> RERIPVEADFLYAYSTVPGYYSWRTTMTG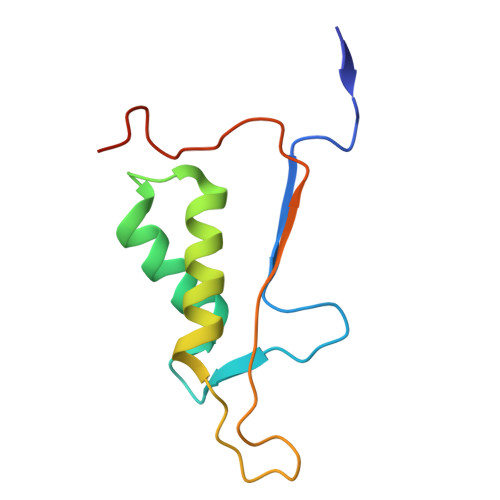SWFIQSLCEMMTKYGSELELLQIMTRVNHKVALDFESTSNMPGFDAKKQIPCIVSMLTKEMYFTPLEHHHHHH> GLAEKLVPAKKVKNGVLYKSGHIKVSNVRCSYPHLDKPYGGEDGGEPKYSITLLMPKDTHGAIKKIIDEQIELTKKNHKTGALKVAPSMLFIKDGDVDFPDKPECEGMWVISARESTRPDVLNMEREELESPNEIAEEIYGGCWVSSVIRPWSQENKYGKRINANLLSVLKRKDDEPFG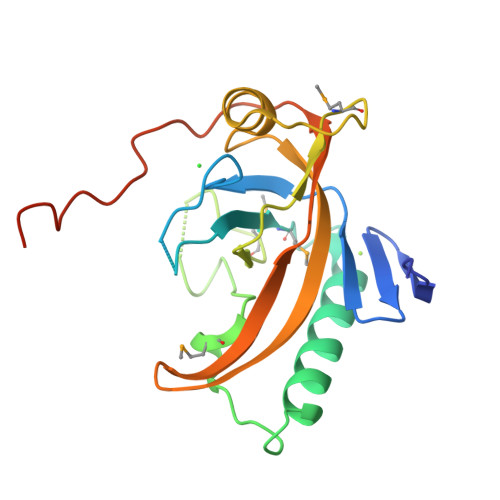EGRVDTSDAYDEDEDEWDEDEV> MPSRAEDYEVLYTIGTGSYGRCQKIRRKSDGKILVWKELDYGSMTEAEKQMLVSEVNLLREL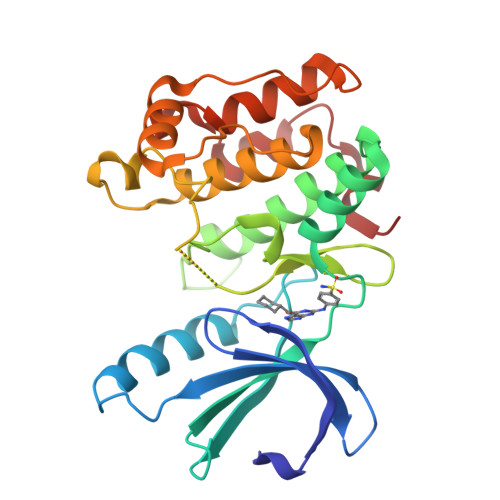KHPNIVRYYDRIIDRTNTTLYIVMEYCEGGDLASVITKGTKERQYLDEEFVLRVMTQLTLALKECHRRSDGGHTVLHRDLKPANVFLDGKQNVKLGDFGLARILNHDTSFAKAFVGTPYYMSPEQMNRMSYNEKSDIWSLGCLLYELCALMPPFTAFSQKELAGKIREGKFRRIPYRYSDELNEIITRMLNLKDYHRPSVEEILENPLILEHHHHHH>[7x]MAIITPALISALKTSFQKHFQDALATAPSTYLQVATVIPSTTASNTYGWLGQFPKLREWIGQRVIKDMAAQGYQITNKLFESTVGVKRTDIEDDNLGVYGPLMQEMGRAAGAHPDELVFALLKAGNANLCYDGQNFFDTDHPVYPNVDGTGTATTVSNLFAPAADPGAAWYLLDTSRSLKPLIYQERMKPSFTSMTKEDDEQVFMADEYRYGVRSRCNVGFGFWQLAAMSTEELNQVNFEKVYDAMRNQKADGGRPLDIRPNLLVVPTTLRSKAKEVVGVQRLANGADNPNFELVQVLDTAWLN

Bacteriophage Casadabanvirus JBD30, from the order Caudoviricetes, is a temperate phage that infects the bacterium Pseudomonas aeruginosa. The virion of bacteriophage JBD30 is composed of an icosahedral capsid, long flexible non-contractile tail, and a baseplate. Using its baseplate, JBD30 attaches to Pseudomonas aeruginosa via the bacterial type IV pilus, whose subsequent retraction brings the phage to the bacterial cell surface.

The icosahedral capsid of bacteriophage JBD30 is built from 415 copies of major capsid proteins organised in a T7 laevo lattice. The classification, performed as a part of the single-particle reconstruction, identified two classes of JBD30 capsids. One of them contained minor capsid proteins whereas the other lacked them. The major capsid protein of JBD30 has the canonical HK-97 fold common to tailed bacteriophages and many other viruses. The major capsid protein can be divided into the N-terminal arm, axial domain, peripheral domain, extended loop, and axial loops. The capsid of JBD30 is formed by pentamers and hexamers of major capsid proteins. Contacts between the pentamers and hexamers are stabilized by the interactions of extended loops, peripheral domains, and N-terminal arms. The extended loop of the major capsid protein stretches over the peripheral domain of the neighbouring subunit positioned clockwise in the same hexamer or pentamer. The three peripheral domains around threefold and pseudo-threefold axes connect either three hexamers, or two hexamers and one pentamer via interactions of α5 helices to form a phenylalanine lock (Phe192). The N-terminal arm extends from the major capsid protein core, protrudes towards the neighbouring capsomer, and forms a small hook that reaches above the spine α-helix.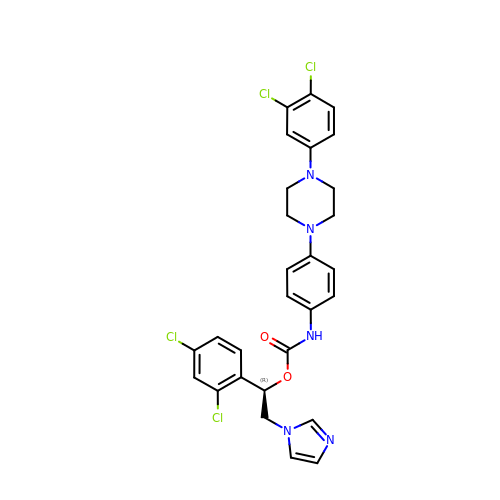(1R)-1-(2,4-dichlorophenyl)-2-(1H-imidazol-1-yl)ethyl {4-[4-(3,4-dichlorophenyl)piperazin-1-yl]phenyl}carbamate | C28 H25 Cl4 N5 O2 | RKYWJGOKHMLHHS-MHZLTWQESA-N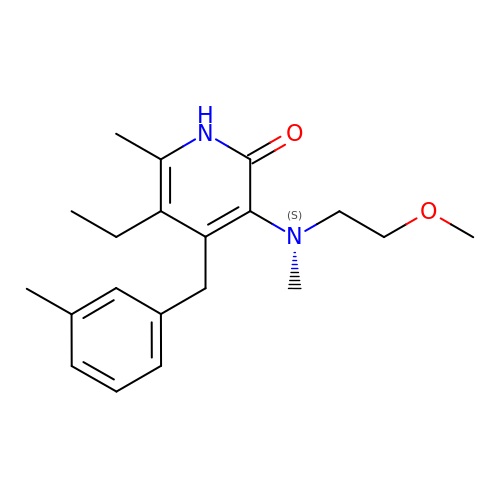5-ETHYL-3-[(2-METHOXYETHYL)METHYLAMINO]-6-METHYL-4-(3-METHYLBENZYL)PYRIDIN-2(1H)-ONE | C20 H28 N2 O2 | USWKTQVAABDFSY-UHFFFAOYSA-N(5R)-N-(1-{2-[4-(2-methoxyethyl)piperazin-1-yl]ethyl}-1H-pyrazol-3-yl)-5,8-dimethyl-9-phenyl-6,8-dihydro-5H-pyrazolo[3,4-h]quinazolin-2-amine | C29 H37 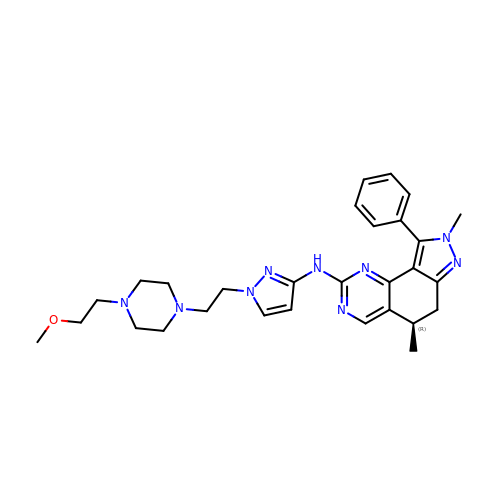N9 O | PHQDLOFSIWRQJZ-OAQYLSRUSA-N> ATRRYYLGAVELSWDYMQSDLGELPVDARFPPRVPKSFPFNTSVVYKKTLFVEFTDHLFNIAKPRPPWMGLLGPTIQAEVYDTVVITLKNMASHPVSLHAVGVSYWKASEGAEYDDQTSQREKEDDKVFPGGSHTYVWQVLKENGPMASDP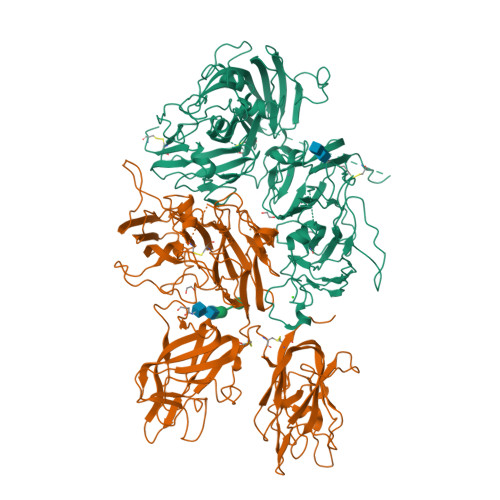LCLTYSYLSHVDLVKDLNSGLIGALLVCREGSLAKEKTQTLHKFILLFAVFDEGKSWHSETKNSLMQDRDAASARAWPKMHTVNGYVNRSLPGLIGCHRKSVYWHVIGMGTTPEVHSIFLEGHTFLVRNHRQASLEISPITFLTAQTLLMDLGQFLLFCHISSHQHDGMEAYVKVDSCPEEPQLRMKNNEEAEDYDDDLTDSEMDVVRFDDDNSPSFIQIRSVAKKHPKTWVHYIAAEEEDWDYAPLVLAPDDRSYKSQYLNNGPQRIGRKYKKVRFMAYTDETFKTREAIQHESGILGPLLYGEVGDTLLIIFKNQASRPYNIYPHGITDVRPLYSRRLPKGVKHLKDFPILPGEIFKYKWTVTVEDGPTKSDPRCLTRYYSSFVNMERDLASGLIGPLLICYKESVDQRGNQIMSDKRNVILFSVFDENRSWYLTENIQRFLPNPAGVQLEDPEFQASNIMHSINGYVFDSLQLSVCLHEVAYWYILSIGAQTDFLSVFFSGYTFKHKMVYEDTLTLFPFSGETVFMSMENPGLWILGCHNSDFRNRGMTALLKVSSCDKNTGDYYEDSYEDISAYLLSKNNAIEPRSFSQNSRHPSQNPPVLKRHQ;> REITRTTLQSDQEEIDYDDTISVEMKKEDFDIYDEDENQSPRSFQKKTRHYFIAAVERLWDYGMSSSPHVLRNRAQSGSVPQFKKVVFQEFTDGSFTQPLYRGELNEHLGLLGPYIRAEVEDNIMVTFRNQASRPYSFYSSLISYEEDQRQGAEPRKNFVKPNETKTYFWKVQHHMAPTKDEFDCKAWAYFSDVDLEKDVHSGLIGPLLVCHTNTLNPAHGRQVTVQEFALFFTIFDETKSWYFTENMERNCRAPCNIQMEDPTFKENYRFHAINGYIMDTLPGLVMAQDQRIRWYLLSMGSNENIHSIHFSGHVFTVRKKEEYKMALYNLYPGVFETVEMLPSKAGIWRVECLIGEHLHAGMSTLFLVYSNKCQTPLGMASGHIRDFQITASGQYGQWAPKLARLHYSGSINAWSTKEPFSWIKVDLLAPMIIHGIKTQGARQKFSSLYISQFIIMYSLDGKKWQTYRGNSTGTLMVFFGNVDSSGIKHNIFNPPIIARYIRLHPTHYSIRSTLRMELMGCDLNSCSMPLGMESKAISDAQITASSYFTNMFATWSPSKARLHLQGRSNAWRPQVNNPKEWLQVDFQKTMKVTGVTTQGVKSLLTSMYVKEFLISSSQDGHQWTLFFQNGKVKVFQGNQDSFTPVVNSLDPPLLTRYLRIHPQSWVHQIALRMEVLGCEAQDLY> 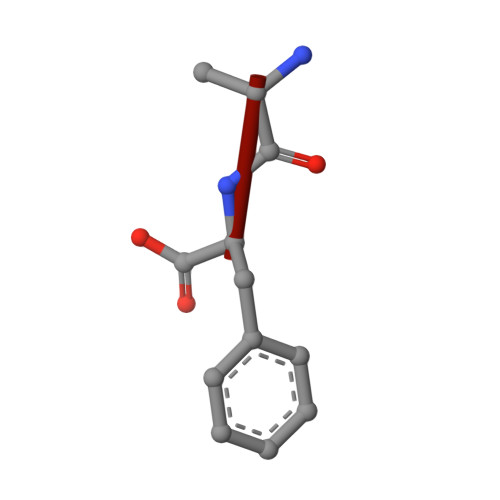AF> MKKLFLVFWWHMHQPLYREPYTGEYLLPWTFFHAVKDYYDMPAYLKDFEIKLNFNLTPVLIDQIQEYAQGKAKDVFLEAIRKDPDDLEKEEVEKLIEFTKLNYEKPIYRFERIRELMNKEKLNREELLDLQTLNLLAWCGRTLRKDLKDLLNKGRNYTQEEKEYVLNKYFEIIKKTLSIYREIKEEGKGSVSTSPYYHPLIPILLNPNCVYETTPNVKIPDFAVSFREDASKHVELAKEKYFEIFGEHPVYMWPPEASVSNEALELYYEKGINMLATDEVILKNSVERASPYLRYYFRELISVFFRDKTLSDLIGFSYHAWNAEDAVRDFIGRLKKIHESVDFQPVVFVVL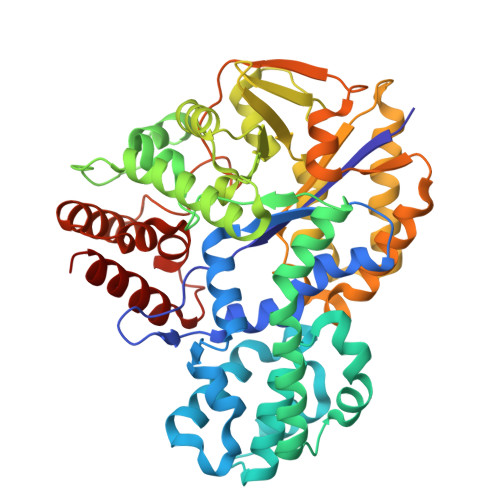DGENCWEYYEENGIPFLEKLYSTLEKEEWIETLTLEEAMRKEDVKTEVIESVKAGTWFDGNFLKWIGNKEKNEYWKILIEAKKKAKNDYILVAEGSDWFWWQGEEKAPFVEVFDKLFRSFVRRAQE> XXXXXXXXXXXXXXXXXXXXXXXXXXXXXXXXXXXXXXXXXXXXXXXXXXXXXXXXXXXXXXXXXXXXXXXXXXXXXXXXXXXXXXXXXXXXXXXXXXXXXXXXXXXXXXXXXXXXXXXXXXXXXXXXXXXXXXXXXXXXXXXXXXXXXXXXXXXXXXXXXXXXXXXXXXXXXXXXXXXXXXXXXXXXXXXXXXXXXXXXXXXXXXXXXXXXXXXXXXXXXXXXXXXXXXXXXXXXXXXXXXXXXXXXXXXXXXXXXXXXXXXXXXXXXXXXXXXXXXXXXXXXXXXXXXXXXXXXXXXXXXXXXXFSTNFRDTVDILVGWHIDHTQKPSLTQQVSGWLQSLEPFWVADLAFSTTLLGQFLEDMEAYAEDLSHVASGESVDEDVPPPSVSLPKLAALLRVFSTVVRSIGERFSPIRGPPITEAYVTDVLYRVMRCVTAANQVFFSEAVLTAANECVGVLLGSLDPSMTIHCDMVITYGLDQLENCQTCGTDYIISVLNLLTLIVEQINTKLPSSFVEKLFIPSSKLLFLRYHKEKEVVAVAHAVYQAVLSLKNIPVLETAYKLILGEMTCALNNLLHSLQLPEACSEIKHEAFKNHVFNVDNAKFVVIFDLSALTTIGNAKNSLIGMWALSPTVFALLSKNLMIVHSDLAVHFPAIQYAVLYTLYSHCTRHDHFISSSLSSSSPSLFDGAVISTVTTATKKHFSIILNLLGILLKKDNLNQDTRKLLMTWALEAAVLMRKSETYAPLFSLPSFHKFCKGLLANTLVEDVNICLQACSSLHALSSSLPDDLLQRCVDVCRVQLVHSGTRIRQAFGKLLKSIPLDVVLSNNNHTEIQEISLALRSHMSKAPSNTFHPQDFSDVISFILYGNSHRTGKDNWLERLFYSCQRLDKRDQSTIPRNLLKTDAVLWQWAIWEAAQFTVLSKLRTPLGRAQDTFQTIEGIIRSLAAHTLNPDQDVSQWTTADNDEGHGNNQLRLVLLLQYLENLEKLMYNAYEGCANALTSPPKVIRTFFYTNRQTCQDWLTRIRLSIMRVGLLAGQPAVTVRHGFDLLTEMKTTSLSQGNELEVTIMMVVEALCELHCPEAIQGIAVWSSSIVGKNLLWINSVAQQAEGRFEKASVEYQEHLCAMTGVDCCISSFDKSVLTLANAGRNSASPKHSLNGESRKTVLSKPTDSSPEVINYLGNKACECYISIADWAAVQEWQNSIHDLKKSTSSTSLNLKADFNYIKSLSSFESGKFVECTEQLELLPGENINLLAGGSKEKIDMKKLLPNMLSPDPRELQKSIEVQLLRSSVCLATALNPIEQDQKWQSITENVVKYLKQTSRIAIGPLRLSTLTVSQSLPVLSTLQLYCSSALENTVSNRLSTEDCLIPLFSEALRSCKQHDVRPWMQALRYTMYQNQLLEKIKEQTVPIRSHLMELGLTAAKFARKRGNVSLATRLLAQCSEVQLGKTTTAQDLVQHFKKLSTQGQVDEKWGPELDIEKTKLLYTAGQSTHAMEMLSSCAISFCKSVKAEYAVAKSILTLAKWIQAEWKEISGQLKQVYRAQHQQNFTGLSTLSKNILTLIELPSVNTMEEEYPRIESESTVHIGVGEPDFILGQLYHLSSVQAPEVAKSWAALASWAYRWGRKVVDNASXXXXXXXXXXXXXXXXXXXXXXXXXXXXXXXXXXXXXXXXXXXXXXXXXXXXXXXXXXXX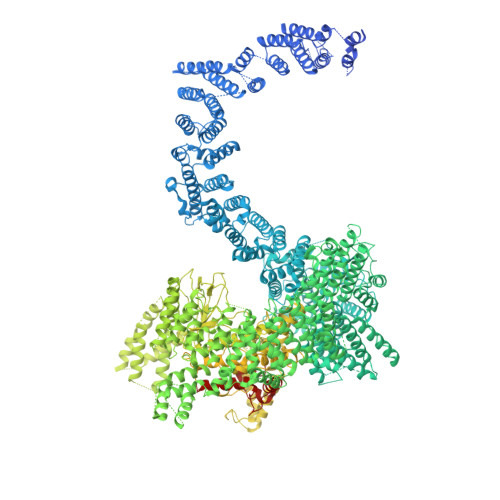XXXXXXXXXXXXXXXXXXXXXXXXXXXXEGVIKVWRKVVDRIFSLYKLSCSAYFTFLKLNAGQIPLDEDDPRLHLSHRVEQSTDDMIVMATLRLLRLLVKHAGELRQYLEHGLETTPTAPWRGIIPQLFSRLNHPEVYVRQSICNLLCRVAQDSPHLILYPAIVGTISLSSESQASGNKFSTAIPTLLGNIQGEELLVSECEGGSPPASQDSNKDEPKSGLNEDQAMMQDCYSKIVDKLSSANPTMVLQVQMLVAELRRVTVLWDELWLGVLLQQHMYVLXXXXXXXXXXXXXXXXXXXXXXXXXXXXXXXXXXXXXXXXXXXXXXXXXXXXXXXXPHEKWFQDNYGDAIENALEKLKXXXXXXXXXXXXXXXXXXXXXXXXXXXXXXXYILRLEEISPWLAAMTNTEIALPGEVSARDTVTIHSVGGTITILPTKTKPKKLLFLGSDGKSYPYLFKGLEDLHLDERIMQFLSIVNTMFATINRQETPRFHARHYSVTPLGTRSGLIQWVDGATPLFGLYKRWQQREAALQAQKAQDSYQTPQNPGIVPRPSELYYSKIGPALKTVGLSLDVSRRDWPLHVMKAVLEELMEATPPNLLAKELWSSCTTPDEWWRVTQSYARSTAVMSMVGYIIGLGDRHLDNVLIDMTTGEVVHIDYNVCFEKGKSLRVPEKVPFRMTQNIETALGVTGVEGVFRLSCEQVLHIMRRGRETLLTLLEAFVYDPLVDWTAGGEAGFAGAVYGGGGQQAESKQSKREMEREITRSLFSSRVAEIKVNWFKNRDEMLVVLPKLDGSLDEYLSLQEQLTDVEKLQGKLLEEIEFLEGAEGVDHPSHTLQHRYSEHTQLQTQQRAVQEAIQVKLNEFEQWITHYQAAFNNLEATQLASLLQEISTQMDLGPPSYVPATAFLQNAGQAHLISQCEQLEGEVGALLQQRRSVLRGCLEQLHHYATVALQYPKAIFQKHRIEQWKTWMEELICNTTVERCQELYRKYEMQYAPQPPPTVCQFITATEMTLQRYAADINSRLIRQVERLKQEAVTVPVCEDQLKEIERCIKVFLHENGEEGSLSLASVIISALCTLTRRNLMMEGAASSAGEQLVDLTSRDGAWFLEELCSMSGNVTCLVQLLKQCHLVPQDLDIPNPMEASETVHLANGVYTSLQELNSNFRQIIFPEALRCLMKGEYTLESMLHELDGLIEQTTDGVPLQTLVESLQAYLRNAAMGLEEETHAHYIDVARLLHAQYGELIQPRNGSVDETPKMSAGQMLLVAFDGMFAQVETAFSLLVEKLNKMEIPIAWRKIDIIREARSTQVNFFDDDNHRQVLEEIFFLKRLQTIKEFFRLCGTFSKTLSGSSSLEDQNTVNGPVQIVNVKTLFRNSCFSEDQMAKPIKAFTADFVRQLLIGLPNQALGLTLCSFISALGVDIIAQVEAKDFGAESKVSVDDLCKKAVEHNIQIGKFSQLVMNRATVLASSYDTAWKKHDLVRRLETSISSCKTSLQRVQLHIAMFQWQHEDLLINRPQAMSVTPPPRSAILTSMKKKLHTLSQIETSIATVQEKLAALESSIEQRLKWAGGANPALAPVLQDFEATIAERRNLVLKESQRASQVTFLCSNIIHFESLRTRTAEALNLDAALFELIKRCQQMCSFASQFNSSVSELELRLLQRVDTGLEHPIGSSEWLLSAHKQLTQDMSTQRAIQTEKEQQIETVCETIQNLVDNIKTVLTGHNRQLGDVKHLLKAMAKDEEAALADGEDVPYENSVRQFLGEYKSWQDNIQTVLFTLVQAMGQVRSQEHVEMLQEITPTLKELKTQSQSIYNNLVSFASPLVTDATNECSSPTSSATYQPSFAAAVRSNTGQKTQPDVMSQNARKLIQKNLATSADTPPSTVPGTGKSVACSPKKAVRDPKTGKAVQERNSYAVSVWKRVKAKLEGRDVDPNRRMSVAEQVDYVIKEATNLDNLAQLYEGWTAWV> APLLLYANRRDLRLVDATNGKENATIVVGGLEDAAAVDFVFSHGLIYWSDVSEEAIKRTEFNKTESVQNVVVSGLLSPDGLACDWLGEKLYWTDSETNRIEVSNLDGSLRKVLFWQELDQPRAIALDPSSGFMYWTDWGEVPKIERAGMDGSSRFIIINSEIYWPNGLTLDYEEQKLYWADA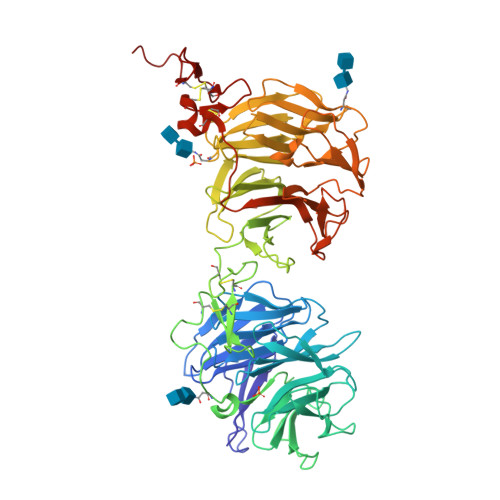KLNFIHKSNLDGTNRQAVVKGSLPHPFALTLFEDILYWTDWSTHSILACNKYTGEGLREIHSDIFSPMDIHAFSQQRQPNATNPCGIDNGGCSHLCLMSPVKPFYQCACPTGVKLLENGKTCKDGATELLLLARRTDLRRISLDTPDFTDIVLQLEDIRHAIAIDYDPVEGYIYWTDDEVRAIRRSFIDGSGSQFVVTAQIAHPDGIAVDWVARNLYWTDTGTDRIEVTRLNGTMRKILISEDLEEPRAIVLDPMVGYMYWTDWGEIPKIERAALDGSDRVVLVNTSLGWPNGLALDYDEGKIYWGDAKTDKIEVMNTDGTGRRVLVEDKIPHIFGFTLLGDYVYWTDWQRRSIERVHKRSAEREVIIDQLPDLMGLKATNVHRVIGSNPCAEENGGCSHLCLYRPQGLRCACPIGFELISDMKTCIVPEAFLL>AYMYRSAFSVGLETRVTVPNVPIRFTKIFYNQQNHYDGSTGKFYCNIPGLYYFSYHITVYMKDVKV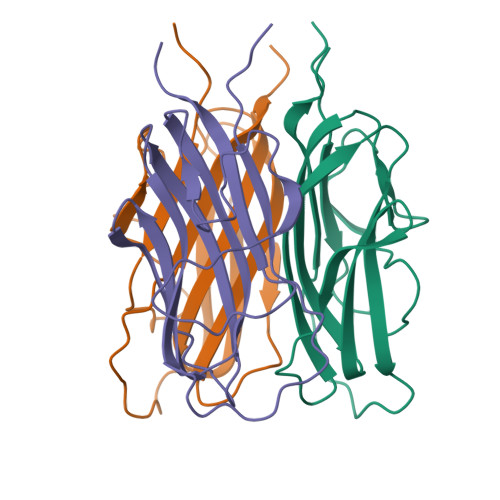SLFKKDKAVLFTYDQYQEKNVDQASGSVLLHLEVGDQVWLQVYGDGDHNGLYADNVNDSTFTGFLLYHDTN[6x]> LAREAALSKIGELASEIFAEFTEGKYSEVVVRAEE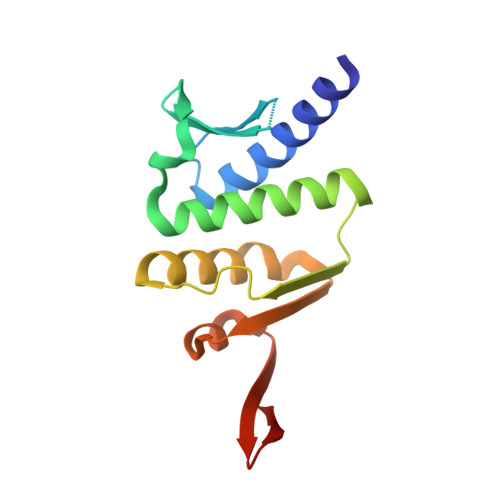NKVRLFVVWEGKERPLTFLRGGERIALGLAFRLAMSLYLAGEISLLILDEPTPYLDEERRRKLITIMERYLKKIPQVILVSHDEELKDAADHVIRISLENGSSKVEVVS We have recently proposed that the trimeric staphylococcal phage encoded dUTPases (Duts) are signaling molecules that act analogously to eukaryotic G-proteins, using dUTP as a second messenger. To initiate the SaPI cycle, a specific phage-encoded protein binds to the SaPI-encoded repressor Stl, acting as an antirepressor. Both the trimeric and the dimeric phage-encoded Dut proteins are the antirepressor proteins for a subset of SaPIs, including SaPIbov1, SaPIbov5 or SaPIov1 (8–10). However, our results analyzing the Dut protein from phage 80α (Dut80α) revealed that motif VI is essential for interaction with the SaPI-encoded Stl repressor, determining the affinity with which the Dut proteins bind to the Stl repressor.

Since motif V is always disordered in the two structurally analyzed mutants (Dut80αD81A and Dut80αY84I), these results reinforce the idea that the Stl:Dut interaction requires the apo form for Stl binding but with the motif V somehow stabilizing the Stl:Dut complex. This idea was partially confirmed with the analysis of the Dut80αG164S protein, which carries a mutation located in the conserved motif V. We have shown in a complementary study that the Dut80αG164S mutant has slightly reduced enzymatic activity but is severely affected in its capacity to induce SaPIbov1. In view of these data, we speculated that this mutant would be able to order the conserved motif V, although the kinetics of this process would be somewhat affected. As anticipated, the crystallographic characterization of the Dut80αG164S mutant showed that this mutant is able to order the motif V in the presence of dUTP, with an identical conformation to that observed in the Dut80αWT protein. In this conformation, the new Ser side chain is exposed to the solvent on the motif V surface. No other differences were observed when this mutant was compared with the structures of the previously characterized Dut80αWT. Interaction analyses with Stl, using BLI, showed that the Dut80αG164S, as Dut80αD81A, had a reduced affinity for the Stl repressor that is further reduced to undetectable binding levels by the nucleotide. Remarkably, the reduction in affinity for Stl observed in the Dut80αG164S mutant, as previously reported for the Dut80αD81A and Dut80αF165A mutants, is explained by an increment in the dissociation rate constant with null or low impact in the association rate constant. In summary, these results support our proposed double role for motif V as the switch and recognition element. On one hand, the motif V conformation induced by the dUTP would interfere in Stl binding (dUTP decreases association rate); on the other, an alternative conformation of this motif is implicated in complex stabilization (deletion or mutations affecting this motif increase dissociation rate).

> MTNTLQVKLLSKNARMPERNHKTDAGYDIFSAETVVLEPQEKAVIKTDVAVSIPEGYVGLLTSRSGVSSKTHLVIETGKIDAGYHGNLGINIKNDHEDDKMQTIFLRNIDNEKIFEKERHLYKLGSYRIEKGERIAQLVIVPIWTPELKQVEEFESVSERGEKSFGSSGV L-THIALYSINE 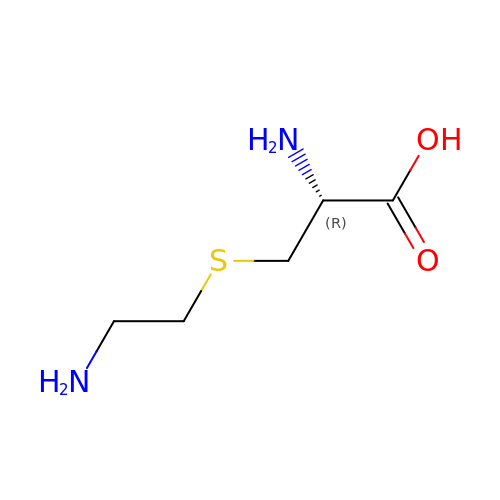| C5 H12 N2 O2 S | GHSJKUNUIHUPDF-BYPYZUCNSA-N> HHHHHHHHGSSLEVLFQGPAVASADGDAPSPVSVSASAATKGPSSSSVLTFQQAIQRLQDYWASVGCAVMQCSNTEVGAGTMNPLTFLRVLGPEPWNVAYVEPSIRPDDSRYGDNPNRLQRHTQFQVILKPDPGNSQDLFLHSLSALGINVREHDIRFVEDNWESPVLGAWGLGWEVWMDGMEITQFTYFQQSGSLPLLPVSVEITYGLERILMSLQGVDHFKNIQYTKGITYGELFLENEKEMSAYYLEHANVDNIQKHFDDFEEEARSLLSLWLPIPAYDHVLKASHAFNILDSRGFVGVTERARYFGRMRSLARQCAQLWVKTRENLGYPLGTYQESNLIYPHVSEKPSRKGVVGQPRAFVLEIGTEELPPHDVIEATKQLEKSLIQILEKRRLSHGKVRSYGTPRRLAVVVENLNMKQMEEEIELRGPPVAKAFDQEGRPTKAAEGFCRKNNVPIDSLYRRTDGKTEYIYARVKESARFADEVLTEDLPTIISGISFPKSMRWNSNIVFSRPIRWIFALHGDLIVPFCFAGISSGNQSCGLRNSSLANFKVEAAELYLHTLEKAGILIDMQERKQRILHDSSILAEGVGGDIIAPDSLVQEVINLVEAPMPIIGRYDVSFLALPKDVLITVMQKHQKYFPVTSKTMGNLLPCFITVANGAIKEEVVRKGNEAVLRARYEDAKFFYKMDTQKKLSEFRDQLSSILFHERLGTMLDKMKRVENTVAEVALLLGINEKMIPAIKDAAALAMSDLATNIVTEFTSLAGIMARHYALRDGLSEQIAEALFEITLPRFSGDVFPKTDPGIVLAVTDRLDSLVGLFGAGCQPSSTNDPFGLRRISYGLVQILVENKKN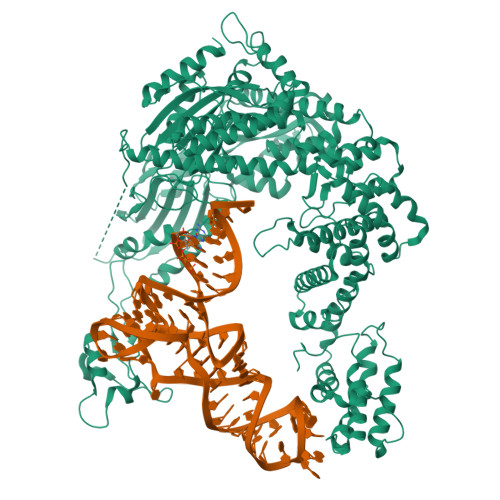FDLTKALTLVAEEQPITIDSGVIDEVVQFVTRRLEQLLVDEGINCEIVRSVLIERANCPYLASQTAIEMEAFSRTEDFPKIVEAYSRPTRIIRGKEIGSALEVDASVFEKDEERALWSAYLEVADKIHPGVDIKAFADASLELLQPLEDFFTNVFVMAEDEKVRNNRLALLTKVASLPKGIADLSVLPGF> MASWSHAPKFEKAGSLDSPTFGCTDSPVRRERGQKAVFCGLTSIVWLHRKMQDAFFLVVGSRTCAHLLQAAAGVMIFAEPRFGTAVLEEQDLAGLADAHKELDREVAKLLERRPDIRQLFLVGSCPSEVLKLDLDRAAERLSGLHAPHVRVYSYTGSGLDTTFTQGEDTCLAAMVPTLDTTEAAELIVVGALPDVVEDQCLSLLTQLGVGPVRMLPARRSDIEPAVGPNTRFILAQPFLGETTGALERRGAKRIAAPFPFGEEGTTLWLKAVADAYGVSAEKFEAVTAAPRARAKKAIAAHLETLTGKSLFMFPDSQLEIPLARFLARECGMKTTEIATPFLHKAIMAPDLALLPSNTALTEGQDLEA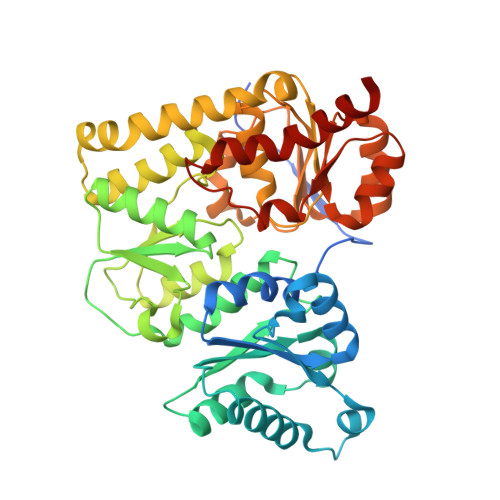QLDRHEAINPDLTVCGLGLANPLEAKGHATKWAIELVFTPVHFYEQAGDLAGLFSRPLRRRALLNGGAA> MH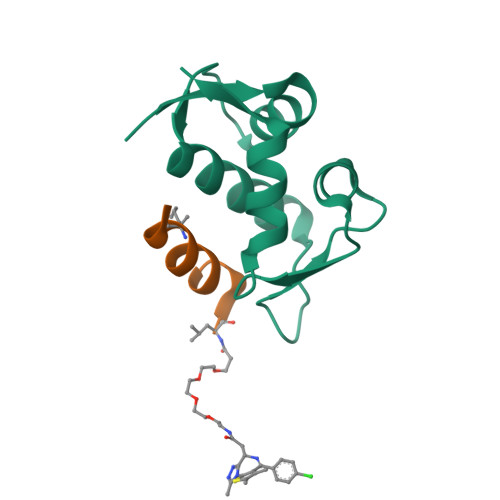HHHHHDDDDKRTTSFSTSAQCSTSDSACRILPGEGTQVHPRAPLLQILKVAGAQEEVFTVKEVMHYLGQYIMMKQLYDKQRQHIVHCHDDPLGELLEVGSFSVKNPSPLYEMLKRNLVILATATTDAAQ;> XXLTFXEYWAQLLSAA(3R,4R,5R)-3-hydroxy-5-(hydroxymethyl)piperidin-4-yl 4-O-beta-D-glucopyranosyl-beta-D-glucopyranoside | C18 H33 N O13 | 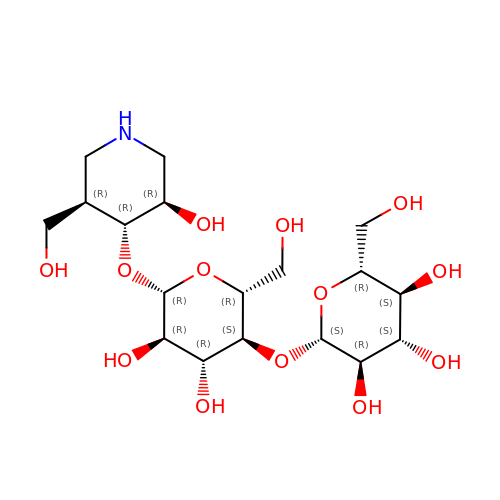ZIMIYDWQNDRGNF-IONZOCAKSA-N> MPLFKFAIDVQYRSNVRDPRGETIERVLREEKGLPVKKLRLGKSIHLEVEAENKEKAYEIVKKACEELL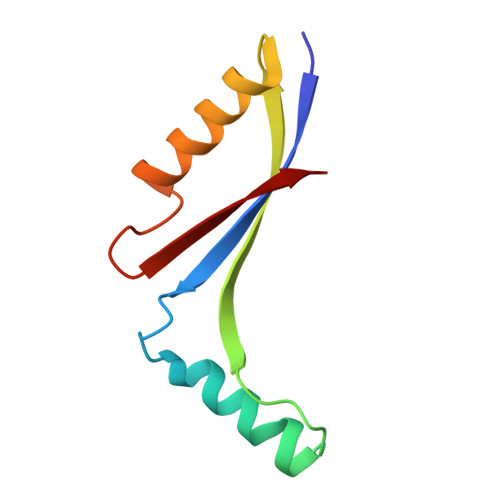VNPVVEEYEVREL>[3x]GSEDLIDGIIFAANYLGSTQLLSERNPSKNIRMMQAQEAVSRVKRMQKAAKIKKKA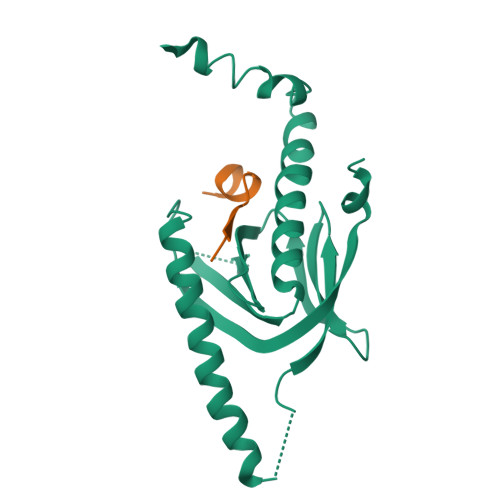NSEGDAQTLTEVDLFISTQRIKVLNADTQETMMDHALRTISYIADIGNIVVLMARRRMPRSASQDCIETTPGAQEGKKQYKMICHVFESEDAQLIAQSIGQAFSVAYQEFLRANGINPEDLSQKEYSDIINTQE;>[3x]QNGYENPTYKFFEQ The conserved aspartate-specific solute-binding protein (SBP) GlnH links extracellular amino acid concentration to PknG activity via the periplasmic transmembrane protein GlnX, thereby controlling glutamate metabolism in Mycobacterium spp. GlnH belongs to the solute-binding protein family, specifically the polar amino acid binding family, which bind to arginine, cysteine, histidine, glutamine, glutamate, and aspartate. The fold of GlnH is related to bacterial solute-binding proteins from ATP transporters and to the sensor domains of glutamate receptors: two lobes close around the Asp ligand in a Venus flytrap-like arrangement. We propose that the amino acid concentration in the periplasm is sensed by GlnH and that protein-protein interaction allows transmission of this information across the membrane via GlnX to activate PknG.

To determine the structural basis of discrimination between higher- and lower-affinity ligands, GlnH was crystallized in the presence of Glu and Asn. Overall, the structures with different ligands bound were similar (Fig. 7A; root mean square deviation [RMSD] = 0.199 Å over 1,727 main-chain atoms). The greatest difference is in loops 99 to 103 and 109 to 113 (DIGSN and DPITG, respectively), which are displaced 2 Å in the Glu- or Asn-bound structures compared to the Asp-bound structure. The conformations of the ligand binding site and positioning of the ligands are similar. Asn is unable to form a hydrogen bond with Trp 232, providing an explanation for the difference in affinity of binding. Addition of aspartate, glutamate, or asparagine increased the thermal stability of GlnH, suggesting that these are ligands for GlnH. Our structures of liganded GlnH represent “closed” conformations.

> LPTPVGMEIMPPQPPLPPDSSSQDCDPTASLRPFATKAEADAAVADIRARGRLIVGLDIGSNLFSFRDPITGEITGFDVDIAGEVARDIFGVPSHVEYRILSAAERVTALQKSQVDIVVKTMSITCERRKLVNFSTVYLDANQRILAPRDSPITKVSDLSGKRVCVARGTTSLRRIREIAPPPVIVSVVNWADCLVALQQREIDAVSTDDTILAGLVEEDPYLHIVGPDMADQPYGVGINLDNTGLVRFVNGTLERIRNDGTWNTLYRKWLTVLGPAPAPPTPRYVD> VDGAADLIDFSVP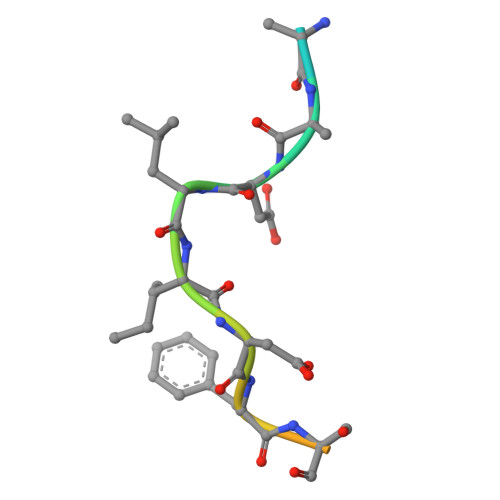TDEY>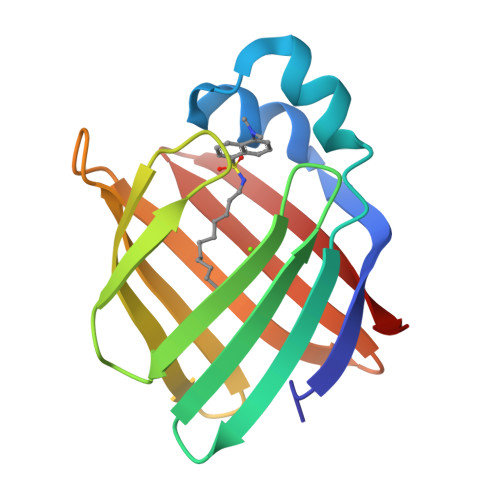AFDSTWKVDRSENYDKFMEKMGVNIVKRKLAAHDNLKLTITQEGNKFTVKESSAFRNIEVVFELGVTFNYNLADGTELRGTWSLEGNKLIGKFKRTDNGNELNTVREIIGDELVQTYVYEGVEAKRIFKKD[4x]> 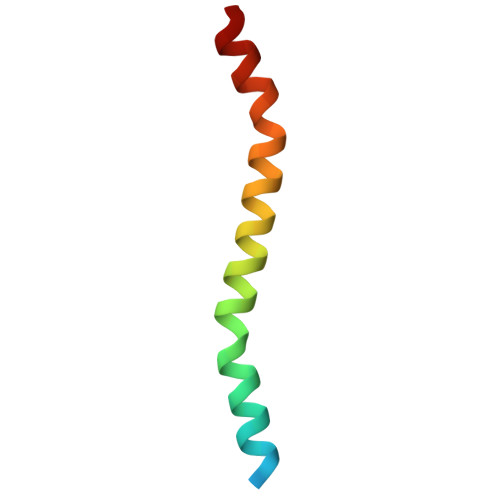GSDYEFLKSWTVEDLQKRLLALDPMMEQEIEEIRQKYQSKRQPILDAIEAK>[4x]ETGWVLAWLRVRRALTLHPAPSALPPDSSSPAVAPELFWGTYRPHVYFGMKTRSPKPLLTGLMWAQQGATPGTPPKLRHTCEQGDGVGPYGWEFHDGRTFGRQHIHDGALRLTTEFVKRPGGQHGGDWSWRVTVEPQASGTPSFPLVSLFFYVVTDGQEVLLPEIGAKGQLKSISGHTSELGDFRLTLLPPTSPGDTVPKHGSYNVFWSSNPGLPQLTDMVKSRLNSWFQHRPPGASPDRYLGLPGSLKWEERGPSGQGQFLIQQ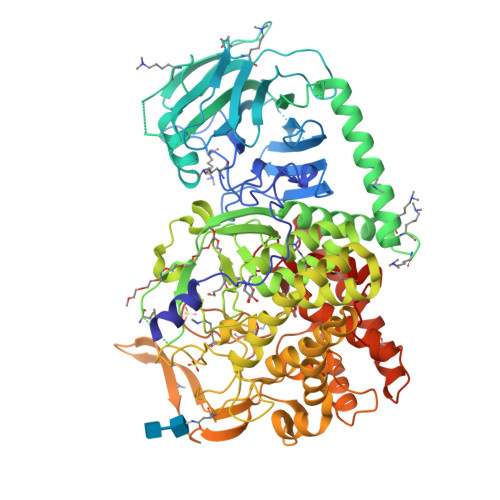VTLKAPFSVEFVFESGSAATGGNQASGRLVGSQLTQALESHAAAFKERFEKTFQLKEKGLSPEEQALGQVALSGLLGGIGYFYGQGLVLPDTSMEGSEQKMDPALFPPVPLFSGVPSRSFFPRGFLWDEGFHQLVVQRWDPHLTREALGHWLGLLNADGWIGREQILGDEARARVPPEFLVQRAAHANPPTLLLPVVHMLEGHDPDDLAFLRKAFPRLHAWFSWLHQSQAGPVPLSYRWRGRDLALPTLLNPKTLPSGLDDYPRASHPSTAERHLDLRCWVALGARVLSQLAEQLGETEAAAELGPLAASLEEPGSLDELHWAPELGVFADFGNHTKAVQLKSRPPQGLVRVVGRPPPRLQYVDALGYVSLFPLLLQLLDPSSPRLGPLLDVLADSRHLWSPFGLRSLSASSLFYKQRNTEHDPPYWRGAVWLNINYLALGALHHYGHVEGPHKVQAAKLYHELRANVVRNVRQQYQATGFLWEQYSDQDGRGMGCRPFQGWTSLVLLIMAEEYASWSHPQFEKHHHHHH>MSRDLQNHLLFETATEVANRVGGIYSVLKSKAPITVAQYKDHYHLIGPLNKATYQNEVDILDWKKPEAFSDEMRPVQHALQTMESRGVHFVYGRWLIEGAPKVILFDLDSVRGYSNEWKGDLWSLVGIPSPENDFETNDAILLGYTVAWFLGEVAHLDS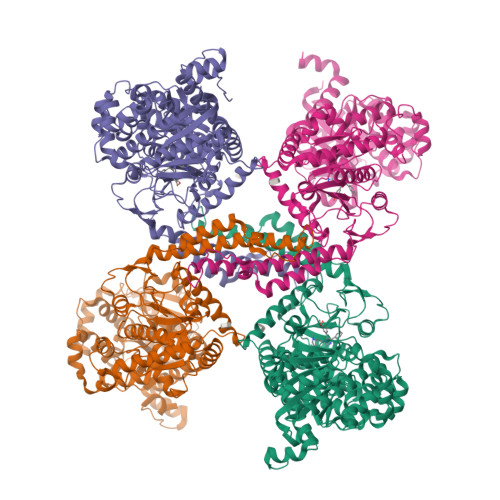QHAIVAHFHEWLAGVALPLCRKRRIDVVTIFTTHATLLGRYLCASGSFDFYNCLESVDVDHEAGRFGIYHRYCIERAAAHSADVFTTVSQITAFEAEHLLKRKPDGILPNGLNVIKFQAFHEFQNLHALKKEKINDFVRGHFHGCFDFDLDNTLYFFIAGRYEYKNKGADMFIEALARLNYRLKVSGSKKTVVAFIVMPAKNNSFTVEALKGQAEVRALENTVHEVTTSIGKRIFDHAIRYPHNGLTTELPTDLGELLKSSDKVMLKRRILALRRPEGQLPPIVTHNMVDDANDLILNKIRQVQLFNSPSDRVKMIFHPEFLNANNPILGLDYDEFVRGCHLGVFPSYYEPWGYTPAECTVMGVPSITTNVSGFGSYMEDLIETNQAKDYGIYIVDRRFKAPDESVEQLVDYMEEFVKKTRRQRINQRNRTERLSDLLDWKRMGLEYVKARQLALRRGYPDQFRELVGEELNDSNMDALAGGKKLKVARPLSVPGSPRDLRSNSTVYMTPGDLGTLQEVNNADDYFSLGVNPAADDDDDGPYADDS[4x]>GSHMLEDPMSFPKGFLWGAATASYQIEGAWNEDGKGESIWDRFTHQKRNILYGHNGDVACDHYHRFEEDVSLMKELGLKAYRFSIAWTRIFPDGFGTVNQKGLEFYDRLINKLVENGIEPVVTLYHWDLPQKLQDIGGWANPEIVNYYFDYAMLVINRYKDKVKKWITFNEPYCIAFLGYFHGIHAPGIKDFKVAMDVVHSLMLSHFKVVKAVKENNIDVEVGITLNLTPVYLQTERLGYKVSEIEREMVSLSSQLDNQLFLDPVLKGSYPQKLLDYLVQKDLLDSQKALSMQQEVKENFIFPDFLGINYYTRAVRLYDENSSWIFPIRWEHPAGEYTEMGWEVFPQGLFDLLIWIKESYPQIPIYITENGAAYNDIVTEDGKVHDSKRIEYLKQHFEAARKAIENGVDLRGYFVWSLMDNFEWAMGYTKRFGIIYVDYETQKRIKKDSFYFYQQYIKENS[2x]

Bgl1 catalyses the final step of in the decomposition of cellulose, an unbranched glucose polymer that has attracted the attention of researchers in recent years as it is the most abundant renewable source of reduced carbon in the biosphere. Bgl1 is a member of glycosyl hydrolase family 1 (GH1 superfamily, EC 3.2.1.21) and the results showed that the 3D structure of Bgl1 follows the overall architecture of the GH1 family, with a classical (β/α)8 TIM-barrel fold. Bgl1 has a half-life of 250 h at 60°C and it has been shown to be a thermostable enzyme with a broad substrate specificity and saccharification ability that efficiently hydrolyses cellooligosaccharides to glucose. The catalytic site residues of the enzyme are two glutamic acid residues, Glu163 and Glu361, as in other enzymes that belong to the same family.

The crystal structures of Bgl1 from the thermophilic bacterium C. saccharo­lyticus and its complex with glucose were determined at 1.47 and 1.95 Å resolution, respectively. In the case of the Bgl1 complex, the overall structure is the same as that of Bgl1. Superposition of the molecules in the asymmetric unit of the Bgl1 complex structure onto the Bgl1 structure showed that the r.m.s.d. on Cα atoms (453 residues) is 0.32 Å and that on secondary-structure elements (905 residues) is 0.36 Å. Comparison of these two structures showed that the residues lining the catalytic site of the enzyme have the same conformation, except for the side chain of Glu163, the χ3 torsion angle of which rotates by ∼30°, and a negligible change of Asn219, the χ1 torsion angle of which rotates by ∼15° to optimize the interaction with glucose. The crystal structure of the enzyme also includes a chlorine ion in the same position as in the Bgl1 structure and a total of two molecules of 1PE (also present as PEG in Bgl1) and one molecule of PEG (bound very close to the position previously occupied by glycerol in Bgl1), as indicated by the 2Fobs − Fcalc and Fobs − Fcalc electron-density maps. The rest of the differences observed in the vicinity of the active site may be attributed to the glycerol molecule entrapped between the two symmetry-related molecules in Bgl1 that induces changes to the side chain of His324, the torsion angles (χ1 and χ2) of which rotate by ∼78° and 34.1°, respectively, in the presence of GOL504. This change is additionally associated with a change in the side chain of Trp322, which is also subjected to a rotation of the χ2 torsion angle by 131.4°. Calculation of 2Fobs − Fcalc and Fobs − Fcalc electron-density maps showed that at the catalytic site of the enzyme, a glycerol molecule was bound to Bgl1 and interacted with the catalytic residues Glu163 and Glu361, but when lactose was used as substrate analogue, β-d-glucose, the product of the catalytic reaction taking place in the crystal, was bound at the same site.> TIKNFTFFSPNSTEFPVGSNNDGKLYMMLTGMDYRTIRRKDWSSPLNTALNVQYTNTSIIAGGRYFELLNETVALKGDSVNYIHANIDLTQTANPVSLSAETANNSNGVDINNGSGVLKVCFDIVTTS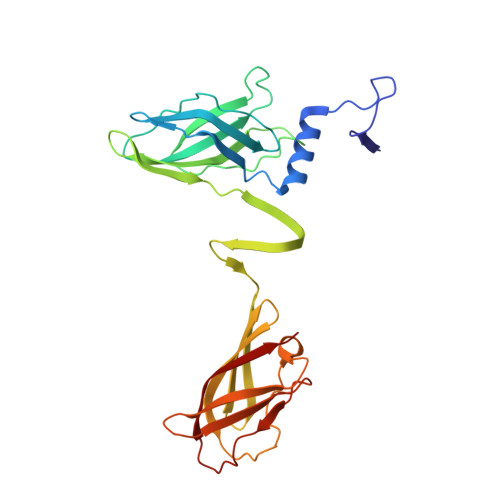GTGVTSTKPIVQTSTLDSISVNDMTVSGSIDVPVQTLTVEAGNGLQLQLTKKNNDLVIVRFFGSVSNIQKGWNMSGTWVDRPFRPAAVQSLVGHFAGRDTSFHIDINPNGSITWWGANIDKTPIATRGNGSYFIK> SMKQYVARLEKDFSLIEHGFKEEEQRALTDYKSNDGEYIKKLAFLAYQSDVYQVRMYAVFLFGYLSKDKEILIF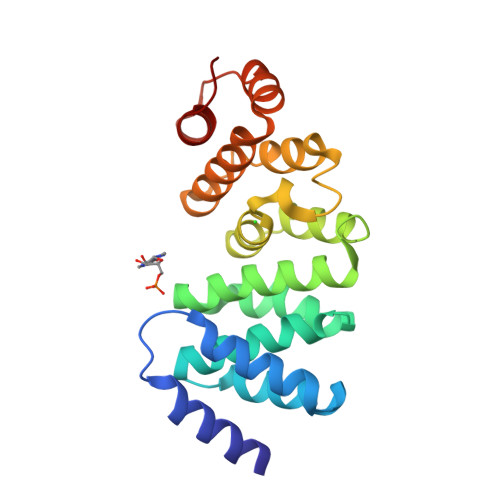MRDEVSKDNNWRVQEVLAKAFDEFCKKIGYKKALPIIDEWLKSSNLHTRRAATEGLRIWTNRPYFKENPNEAIRRIADLKEDVSEYVRKSVGNALRDISKKFPDLVKIELKNWKLESKEINQVYKLASKFIDA>[3x]ATDGSHFDFVIVGGGTAGNTVAGRLAENPNVTVLIVEAGIGNPEDIPEITTPSSAMDLRNSKYDWAYKTTMVRRDDYERIEKPNTRGKTLGGSSSLNYFTWVPGHKATFDQWEEFGGKEWTWDPLVPYLRKSATYHDDPRLY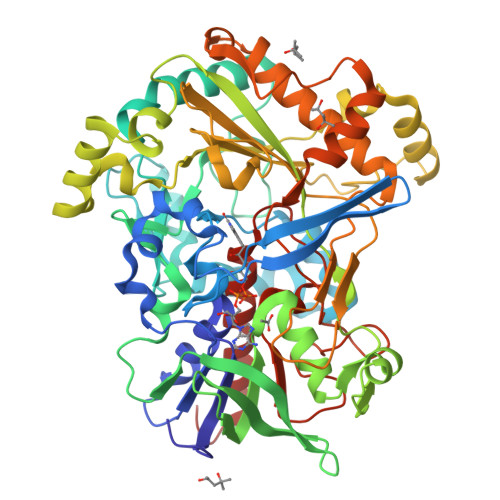SPELEKIGGGGPIPISHAELIDEMAPFRENLTKAWKSMGQPLIENIYDGEMDGLTHCCDTIYRGQRSGSFLFVKNKPNITIVPEVHSKRLIINEADRTCKGVTVVTAAGNELNFFADREVILSQGVFETPKLLMLSGIGPTRELSRHGINTIVDSRHVGQNLMDHPGVPFVLRVKDGFGMDDVLLRHGPKRDAVVSAYNKNRSGPVGSGLLELVGFPRIDKYLEKDAEYRKAKAANGGKDPFSPLGQPHFELDFVCMFGTAFQWHFPTPKTGDHLTVVVDLVRPISDPGEVTLNSADPFQQPNINLNFFANDLDIIAMREGIRFSYDLLFKGEGFKDLVESEYPWEMPLDSDKEMHRAVLDRCQTAFHPTGTARLSKNIDQGVVDPKLKVHGIKKLRVADASVIPIIPDCAIQNSVYAVGEKCADMIKAEHKDLY> AFISSGYNPAKPMENRITDIGPRKFTEFFPPVIAKNAGNWDYHEILEPGILVHVAKNGDKVFTVRCGAARLMSTSHIREACEIAKKFC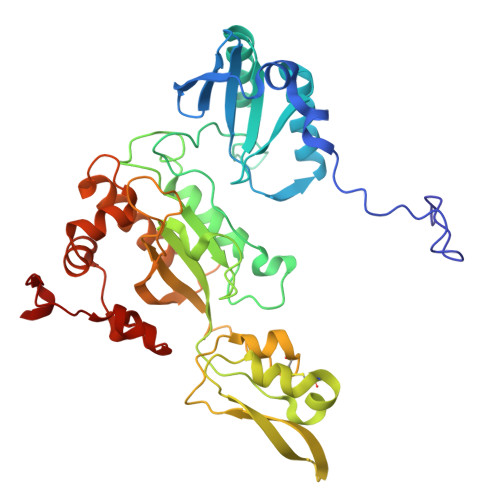NGHLRFTTRNNIEFMVDNEETLKALVADLKTRKFAAGSFKFPIGGTGASISNIVHTQGWVYCHTPATDASGPVKAVMDELFEEFTSMRLPAIVRVSLACCINMCGAVHCSDIGLVGIHRKPPMIDHENLAELCEIPLAVAACPTAAVKPITAEVNGQKVKSVAINNDRCMYCGNCYTMCPALPLSDGTGDGIAIMVGGKISNRIKVPSFSKVVVAFVPNEPPRWPTMAKIVKKIVEVYAEDARKYERIGDWIHRIGWETFYEKTGLEFSHHCIDDFRDPAYYTWRQSTQFKFVSFDS> MSASKEEIA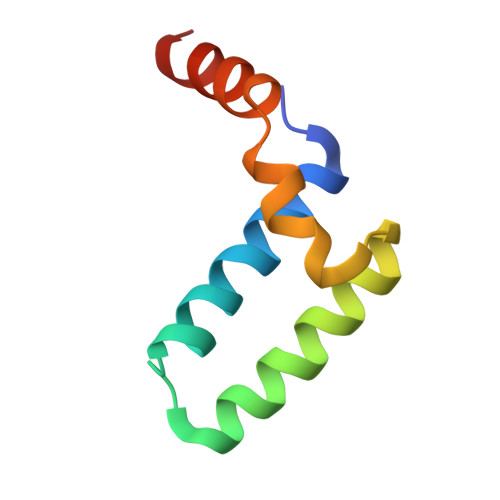ALIVNYFSSIVEKKEISEDGADSLNVAMDCISEAFGFEREAVSGILGKSEFKGQHLADILNSA>MGSSHHHHHHSQDPMSLNLVSEQLLAANGLKHQDLFAILGQLAERRLDYGDLYFQSSYHESWVLEDRIIKDGSYNIDQGVGVRAISGEKTGFAYADQISLLALEQSAQAARTIVRDSGDGKVQTLGAVEHSPLYTSVDPLQSMSREEKLDILRRVDKVAREADKRVQEVTASLSGVYELILVAATDGTLAADVRPLVRLSVSVLVEEDGKRERGASGGGGRFGYEFFLADLDGEVRADAWAKEAVRMALVNLSAVAAPAGTMPVVLGAGWPGVLLHAAVGHGLEGDFNRRGTSVFSGQVGELVASELCTVVDDGTMVDRRGSVAIDDEGTPGQYNVLIENGILKGYMQDKLNARLMGMTPTGNGRRESYAHLPMPRMTNTYMLPGKSTPQEIIESVEYGIYAPNFGGGQVDITSDKFVFSTSEAYLIENGKVTKPVKGATLIGSGIETMQQISMVGNDLKLDNGVGVCGKEGQSLPVGVGQPTLKVDNLTVGGTA[2x];>MALAMKVISQVEAQRKILEEAVSTALELASGKSDGAEVAVSKTTGISVSTRYGEVENVEFNSDGALGITVYHQNRKGSASSTDLSPQAIARTVQAALDIARYTSPDPCAGVADKELLAFDAPDLDLFHPAEVSPDEAIELAARAEQAALQADKRITNTEGGSFNSHYGVKVFGNSHGMLQGYCSTRHSLSSCVIAEENGDMERDYAYTIGRAMSDLQTPEWVGADCARRTLSRLSPRKLSTMKAPVIFANEVATGLFGHLVGAIAGGSVYRKSTFLLDSLGKQILPDWLTIEEHPHLLKGLASTPFDSEGVRTERRDIIKDGILTQWLLTSYSARKLGLKSTGHAGGIHNWRIAGQGLSFEQMLKEMGTGLVV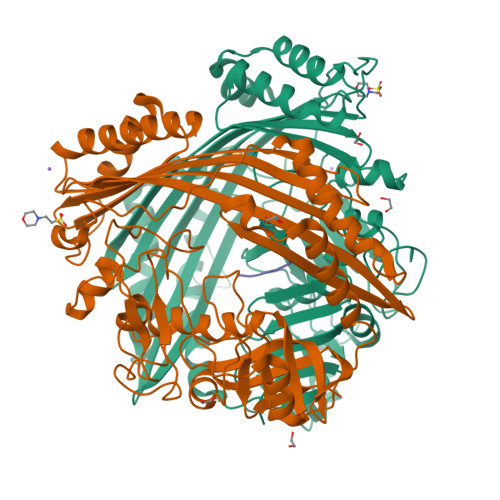TELMGQGVSAITGDYSRGAAGFWVENGEIQYPVSEITIAGNLKDMWRNIVTVGNDIETRSNIQCGSVLLPEMKIAGQ[2x];>VLEDRI[2x]> GPGSELPQMVQQLNSPDQQELQSALRKLSQIASGGNEQIQAVIDAGALPALVQLLSSPNEQIL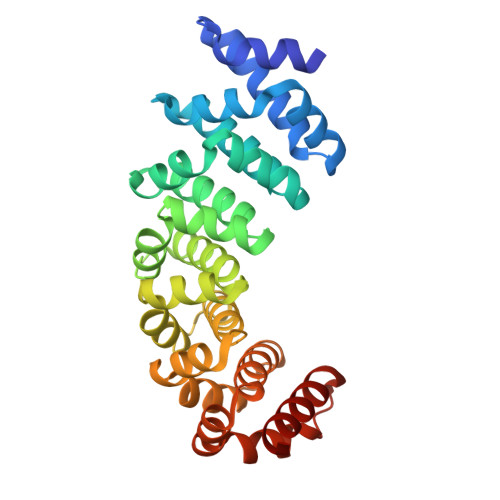QEALWALSNIASGGNEQIQAVIDAGALPALVQLLSSPNEQILQEALWALSNIASGGNEQIQAVIDAGALPALVQLLSSPNEQILQEALWALSNIASGGNEQIQAVIDAGALPALVQLLSSPNEQILQEALWALSNIASGGNEQIQAVIDAGALPALVQLLSSPNEQILQEALWALSNIASGGNEQKQAVKEAGALEKLEQLQSHENEKIQKEAQEALEKLQSH N-[3-(acetylamino)phenyl]-4-chloro-N-[(1S)-1-cyclohexyl-2-(cyclohexylamino)-2-oxoethyl]benzamide | C29 H36 Cl N3 O3 | 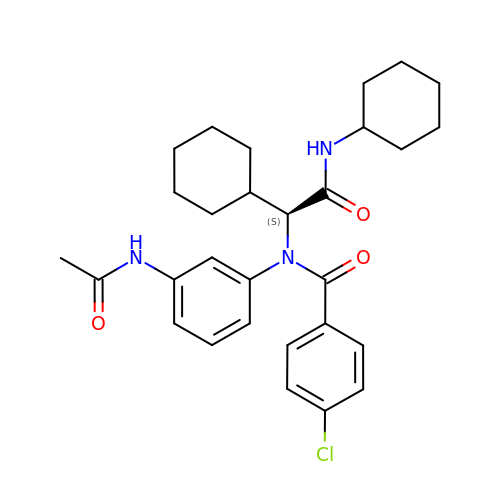GTILSQWOUVGGRG-MHZLTWQESA-N> GGACAUAUAUACGCGUG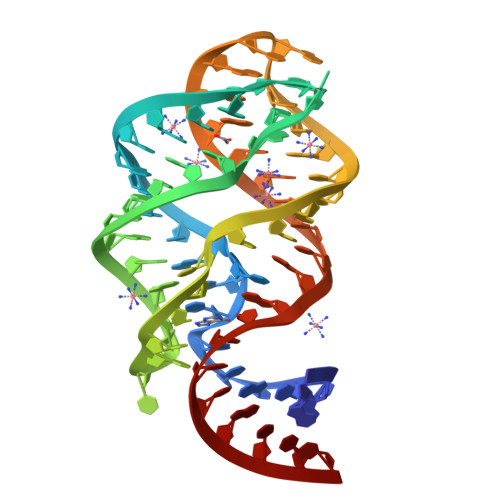GAUAUGGCACGCGAGUUUCUACCGGGCACCGUAAAUGUCCGACUAUGUCC>[60x]MSDEVSSSTDVVSRKRRRHDEGGKALEDIAVHGASEGDGSAPGGSVWQTTDYIALSMVVYRTAIKLRNFVNIRGLTPTEMIVIPWNVMRFYCEYNTGTYGLSGNVHHKNYSMLLACKAHRPTKVGYTLSNLILTSDELVSTGGTLGTTTTFNTSPYMIHSIDDQQCLSKVYPKTDTVWPVSSMRELDYVASTVSGDNAIIPSTIFNKNRYWKQGDDALHFSHDLDLGFWFG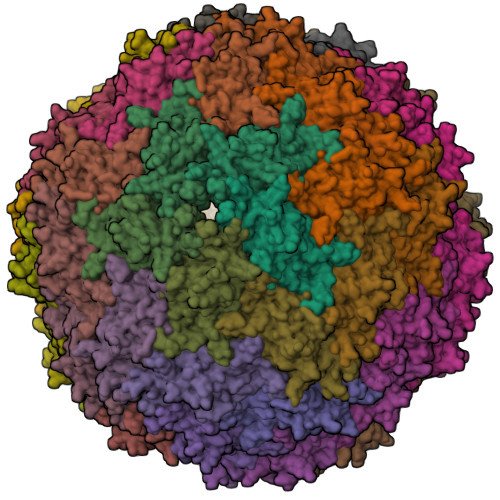SDYGNAYVPQNNDSMNAVGTIPTSKHINVRGVNNRGMAGHYLSFPPIRTNDGQFKLNAQFTLETEIEFEFRLWEQGVQGINSVHTNLNPANDSLWIQSYGSLVSITESKINNIQFGPTCPRVDARNKGGKMSMLFDHH> IAAILVANAKEPCPPENLQLPPRALVGKWYLRTTSPDIFKQVSNITEFYSAHGNDYYGTVTDYSPEYGLEAHRVNLTVSGSTLKFYMNDTHDYDSEYQILAVDKDYFIFYGHPPAAPSGLALIHYR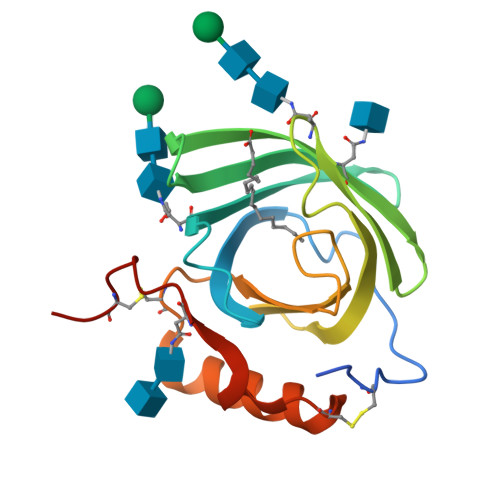QSCPKEDVIKRVKKNLKNVCLDYKYFGNDTSVPCHYVE>[4x]MQFPQLDPATLAAFS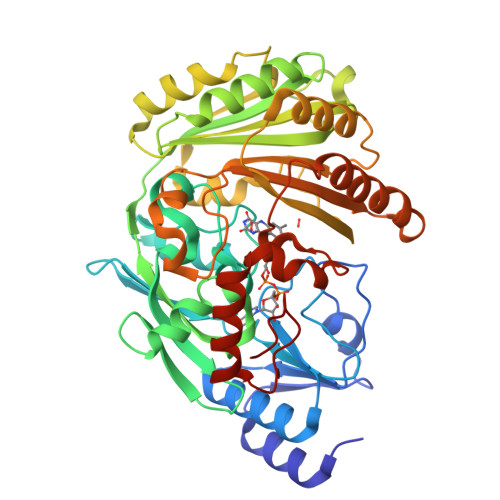AAFRGELIWPSDADYDEARRIWNGTIDRRPALIARCTSTPDVVAAVSFARKSGLLVAVRGGGHSMAGHSVCDGGIVIDLSLMNSIKVSRRLRRARAQGGCLLGAFDTATQAHMLATPAGVVSHTGLGGLVLGGGFGWLSRKYGLSIDNLTSVEIVTADGGVLTASDTENPDLFWAVRGGGGNFGVVTAFEFDLHRVGPVRFASTYYSLDEGPQVIRAWRDHMATAPDELTWALYLRLAPPLPELPADMHGKPVICAMSCWIGDPHEGERQLESILHAGKPHGLTKATLPYRALQAYSFPGAVVPDRIYTKSGYLNELSDEATDTVLEHAADIASPFTQLELLYLGGAVARVPDDATAYPNRQSPFVTNLAAAWMDPTEDARHTAWAREGYRALAGHLSGGYVNFMNPGEADRTREAYGAAKFERLQGVKAKYDPTNLFRLNQNIPPSSP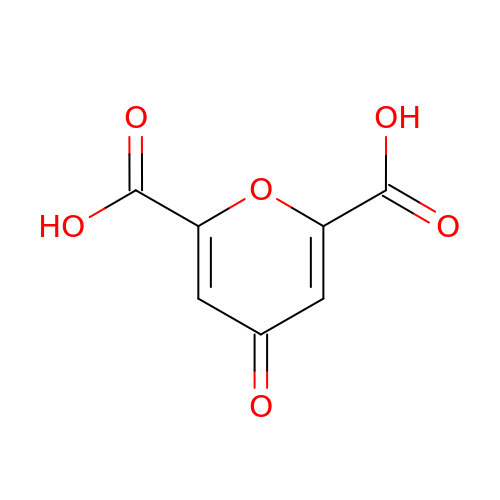4-oxo-4H-pyran-2,6-dicarboxylic acid | C7 H4 O6 | PBAYDYUZOSNJGU-UHFFFAOYSA-N>GAMGSTFLARLNFIWKGFINMPSVAKFVTKAYPVSGSPEYLTEDLPDSIQVGGRISPQTVWDYVEKIKASGTKEICVVRFTPVTEEDQISYTLLFAYFSSRKRYGVAANNMKQVKDMYLIPLGATDKIPHPLVPFDGPGLELHRPNLLLGLIIRQKLK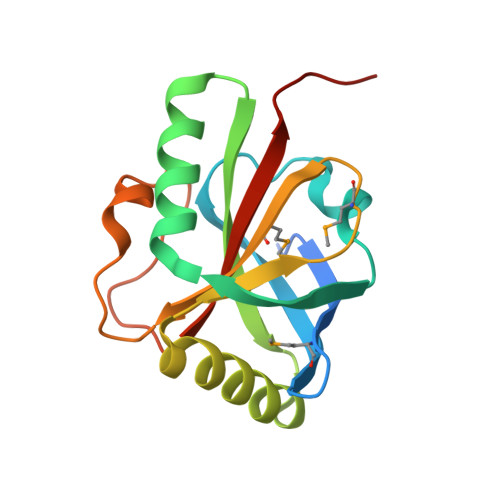RQHS[8x]>[2x]MALSTATKAATDALAANRAPTSVNAQEVHRWLQSFNWDFKNNRTKYATKYKMANETKEQFKLIAKEYARMEAVKDERQFGSLQDALTRLNAGVRVHPKWNETMKVVSNFLEVGEYNAIAATGMLWDSAQAAEQKNGYLAQVLDEIRHTHQCAYVNYYFAKNGQDPAGHNDARRTRTIGPLWKGMKRVFSDGFISGDAVECSLNLQLVGEACFTNPLIVAVTEWAAANGDEITPTVFLSIETDELRHMANGYQTVVSIANDPASAKYLNTDLNNAFWTQQKYFTPVLGMLFEYGSKFKVEPWVKTWDRWVYEDWGGIWIGRLGKYGVESPRSLKDAKQDAYWAHHDLYLLAYALWPTGFFRLALPDQEEMEWFEANYPGWYDHYGKIYEEWRARGCEDPSSGFIPLMWFIENNHPIYIDRVSQVPFCPSLAKGASTLRVHEYNGEMHTFSDQWGERMWLAEPERYECQNIFEQYEGRELSEVIAELHGLRSDGKTLIAQPHVRGDKLWTLDDIKRLNCVFKNPVKAFN;>[2x]MSMLGERRRGLTDPEMAAVILKALPEAPLDGNNKMGYFVTPRWKRLTEYEALTVYAQPNADWIAGGLDWGDWTQKFHGGRPSWGNETTELRTVDWFKHRDPLRRWHAPYVKDKAEEWRYTDRFLQGYSADGQIRAMNPTWRDEFINRYWGAFLFNEYGLFNAHSQGAREALSDVTRVSLAFWGFDKIDIAQMIQLERGFLAKIVPGFDESTAVPKAEWTN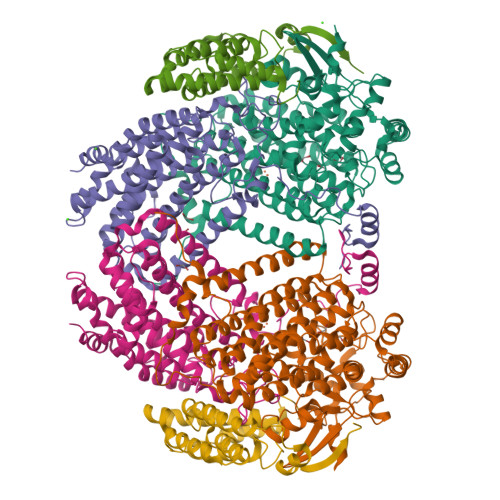GEVYKSARLAVEGLWQEVFDWNESAFSVHAVYDALFGQFVRREFFQRLAPRFGDNLTPFFINQAQTYFQIAKQGVQDLYYNCLGDDPEFSDYNRTVMRNWTGKWLEPTIAALRDFMGLFAKLPAGTTDKEEITASLYRVVDDWIEDYASRIDFKADRDQIVKAVLAGLK;>[2x]MAKLGIHSNDTRDAWVNKIAQLNTLEKAAEMLKQFRMDHTTPFRNSYELDNDYLWIEAKLEEKVAVLKARAFNEVDFRHKTAFGEDAKSVLDGTVAKMNAAKDKWEAEKIHIGFRQAYKPPIMPVNYFLDGERQLGTRLMELRNLNYYDTPLEELRKQRGVRVVHLQSPH> SHHHHHHG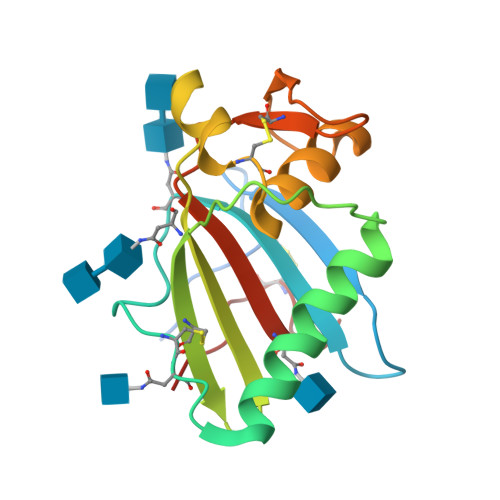GMETLNMTMPLSCTKNNSHHYIMVGNETGLELTLTNTSIINHKFCNLSDAHKKNLYDHALMSIISTFHLSIPNFNQYEAMSCDFNGGKISVQYNLSHSYAGDAANHCGTVANGVLQTFMRMAWGGSYIALDSGRGNWDCIMTSYQYLIIQNTTWEDHCQFSRPS>SRLNRESVIDAALELLNETGIDGLTTRKLAQKLGIEQPTLYWHVKNKRALLDALAVEILARHHDYSLPA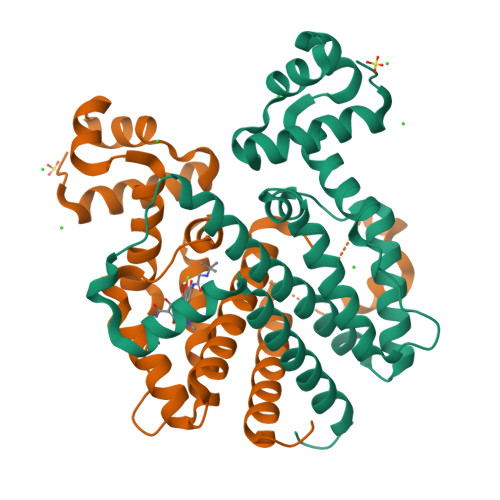AGESWQSFLRNNAMSFRRALLRYRDGAKVHLGTRPDEKQYDTVETQLRFMTENGFSLRDGLYAISAVSHFTLGAVLEQQEHTAALTDRPAAPDENLPPLLREALQIMDSDDGEQAFLHGLESLIRGFEVQLTALLQIV[2x]> 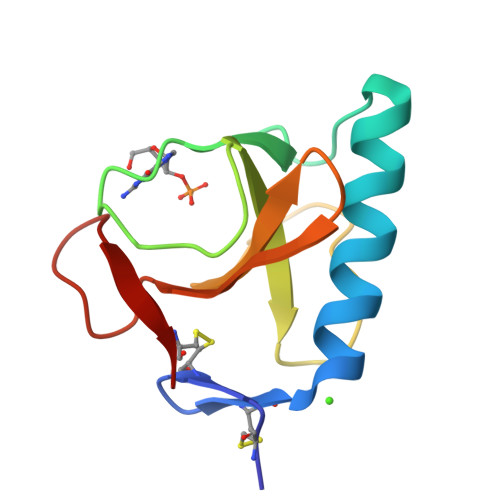ACDYTCGSNCYSSSDVSTAQAAAYKLHEDGETVGSNSYPHKYNNYEGFDFSVSSPYYEWPILSSGDVYSGGSPGADRVVFNENNQLAGVITHTGASGNNFVECT>TPEMPVLENRAAQGDITAPGGARRLTGDQTAALRDSLSDKPAKNIILLIGDGMGDSEITAARNYAEGAGGFFKGIDALPLTGQYTHYALNKKTGKPDYVTDSAASATAWSTGVKTYNGALGVDIHEKDHPTILEMAKAAGLATGNVSTAELQGATPAALVAHVTSRKCYGPSATSEKCPGNALEKGGKGSITEQLLNARADVTLGGGAKTFAETATAGEWQGKTLREQAEARGYQLVSDAASLNSVTEANQQKPLLGLFADGNMPVRWLGPKATYHGNIDKPAV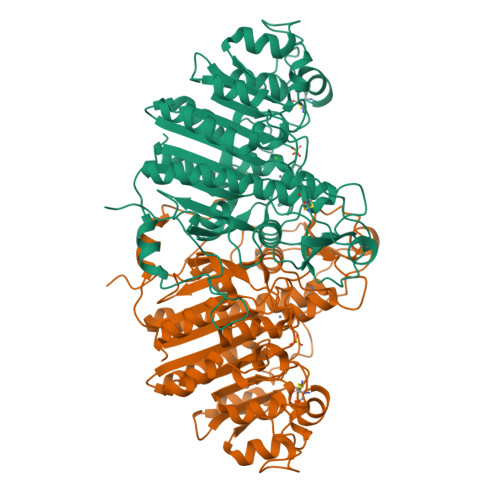TCTPNPQRNDSVPTLAQMTDKAIELLSKNEKGFFLQVEGASIDKQDHAANPCGQIGETVDLDEAVQRALEFAKKEGNTLVIVTADHAHASQIVAPDTKAPGLTQALNTKDGAVMVMSYGNSEEDSQEHTGSQLRIAAYGPHAANVVGLTDQTDLFYTMKAALGLK[2x]The KP32 bacteriophage belongs to the Caudovirales family and can infect multidrug resistant K. pneumoniae isolates. Analysis of the KP32 genome revealed the presence of three tail proteins that are predicted to be involved in the bacterial infection machinery: tail tubular protein A (TTPA), tail tubular protein B (TTPB), and tail fiber protein (TFP). TTPA is a structural protein that is located in the bacteriophage tail core; it is necessary for the adhesion of the phage to the bacterial cell wall, which is a prerequisite for host infection. Interestingly, although TTPA is considered a structural protein, it also possesses the depolymerase activity described in this paper.

All four monomers are folded almost identically. The TTPA molecule consists of 192 amino acid residues; in the electron density map, however, all of the chains have an additional nine expression-plasmid-derived amino acids at the N-terminus (numbered −8 to 0). The electron density maps are interpretable for amino acid residues −8 to 175 of chain B and −8 to 176 for chains C and D. Thus, about 15 residues at the C-termini of chains B, C, and D are not seen in the crystal structure. In chain A, most of the C-terminal part (except for residues 181–184) is visible and forms a well-defined α-helix. The solvent water molecules were classified on the basis of electron density and B factors into 885 fully occupied and 10 half-occupied sites. The structure was refined at a resolution of 1.9 Å to an R factor of 18.3% and an R free of 22.8% in an isotropic mode. However, the TTPA molecule has an additional domain consisting of two antiparallel β-sheets and loops, which lacks in gp11 and gp4. Moreover, the crystallized TTPA molecules adopt a tetrameric structure in which the helical domains are directed toward one another to generate the hydrophobic core, while the loop/β-sheet regions are directed to the outside; thus, there is relatively limited contact between monomers. Our Phyre2 server analysis (confidence 67.3% and identity 21%) showed that the antiparallel β-sheet region (residues 57–99) of TTPA may contain a lectin-like domain; as such domains interact with oligosaccharides, this finding suggests that TTPA could display glucanase activity. We therefore propose that the D121-X-D123 and D151-X-E153 residues of TTPA may be good candidate catalytic residues.

>[4x]SGLVPRGSHMNMQDAYFGSAAELDAVNEMLAAIGESPVTTLDEDGSADVANARRILNRINRQIQSKGWAFNINESATLTPDVSTGLIPFRPAYLSILGGQYVNRGGWVYDKSTGTDTFSGPITVTLITLQDYDEMPECFRQWIVTKASRQFNSRFFGAEDVENSLAQEEMEARMACNEYEMDFGQYNMLDGDAYVQGLIGR>MIPVVYSNLCPVCGGDLESKEIEKHVCFRKKRSLCLFPEDFLLKEFVEFFRKCVGEPRAIQKMWAKRILRKESFAATAPTGVGKTSFGLAMSLFLALKGKRCYVIFPTSLLVIQAAETIRKYAEKAGVGTENLIGYYHGRIPKREKENFMQNLRNFKIVITTTQFLSKHYRELGHFDFIFVDDVDAILKASKNVDKLLHLLGFHYDLKTKSWVGEARGCLMVSTATAKKGKKAELFRQLLNFDIGSSRITVRNVEDVAVNDESISTLSSILEKLGTGGIIYARTGEEAEEIYESLKNKFRIGIVTATKKGDYEKFVEGEIDHLIGTAHYYGTLVRGLDLPERIRFAVFVGCPSFRVTIEDIDSLSPQMVKLLAYLYRNVDEIERLLPAVERHIDEVREILKKVMGKERPQAKDVVVREGEVIFPDLRTYIQGSGRTSRLFAGGLTKGASFLLEDDSELLSAFIERAKLYDIEFKSIDEVDFEKLSRELDESRDRYRRRQEFDLIKPALFIVESPTKARQISRFFGKPSVKVLDGAVVYEIPMQKYVLMVTASIGHVVDLITNRGFHGVLVNGRFVPVYASIKRCRDCGYQFTEDRESCPKCGSENVDNSRSRIEALRKLAHDAEFVIVGTDPDTEGEKIAWDLKNLLSGCGAVKRAEFHEVTRRAILEALESLRDVDENLVKAQVVRRIEDRWIGFVLSQKLWERFNNRNLSAGRAQTLVLGWIIDRFQESRERRKIAIVRDFDLVLEHDEEEFDLTIKLVEEREELRTPLPPYTTETMLSDANRILKFSVKQTMQIAQELFENGLITYH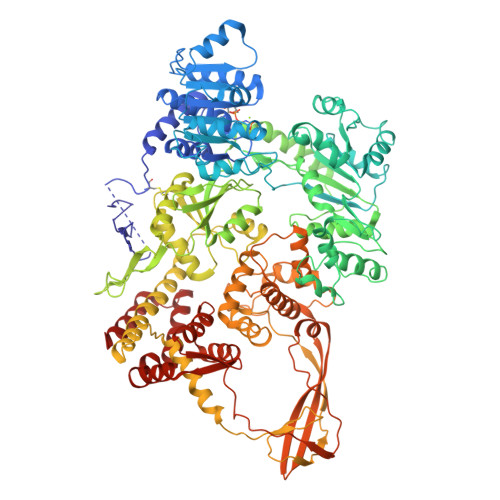RTDSTRVSDVGQRIAKEYLGDDFVGREWGESGAHECIRPTRPLTRDDVQRLIQEGVLVVEGLRWEHFALYDLIFRRFMASQCRPFKVVVKKYSIEFDGKTAEEERIVRAEGRAYELYRAVWVKNELPTGTFRVKAEVKSVPKVLPFTQSEIIQMMKERGIGRPSTYATIVDRLFMRNYVVEKYGRMIPTKLGIDVFRFLVRRYAKFVSEDRTRDLESRMDAIERGELDYLKALEDMYAEIKSID[2x]>[6x]MVVIKDIVAREILDSRGNPTIEVDVSTEGGVFRAAVPSGASTG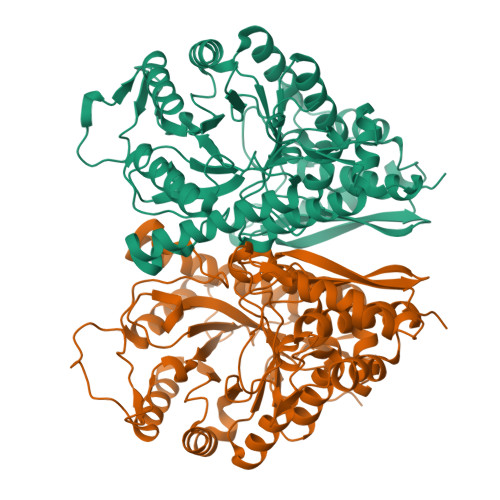IYEALELRDKDPKRYLGKGVLNAVEIVRQEIKPALLGKDPCDQKGIDMLMVEQLDGTKNEWGYSKSKLGANAILGVSIACCRAGAASKGLPLYKYIATLAGKTIDKMVMPVPFFNVINGGEHAGNGLALQEFLIAPVGAPNIREAIRYGSETYHHLKNVIKNKYGLDATNVGDEGGFAPNVATAEEALNLLVEAIKAAGYEGKIKIAFDAAASEFYKQDEKKYDLDYKCKTKNASKHLTGEKLKEVYEGWLKKYPIISVEDPFDQDDFASFSAFTKDVGEKTQVIGDDILVTNILRIEKALKDKACNCLLLKVNQIGSVTEAIEACLLAQKSGWGVQVSHRSGETEDSFIADLVVGLRCGQIKSGSPCRSERLCKYNQLMRIEESLGADCVYAGESFRHPKRSHHHHHH>[4x]AECSVDIQGNDQMQFNTNAITVDKSCKQFCVNLSHPGN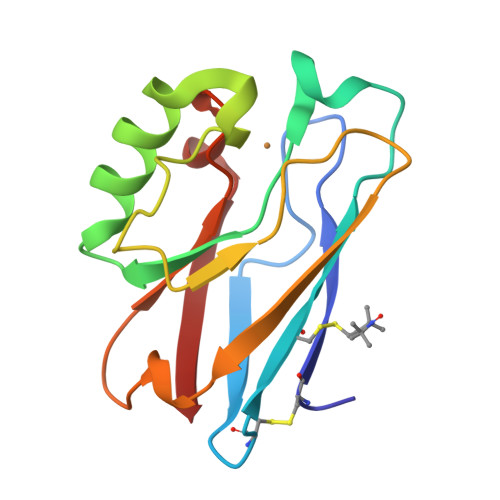LPKNVMGHNWVLSTAADMQGVVTDGMASGLDKDYLKPDDSRVIAHTKLIGSGEKDSVTFDVSKLKEGEQYMFFCTFPGHSALMKGTLTLK> MVSGVGGSGGGRGGGRGGEEEPSSSHTPNNRRGGEQAQSSGTKSLRPRSNTESMSKAIQQYTVDARLHAVFEQSGESGKSFDYSQSLKTTTYGSSVPEQQITAYLSRIQRGGYIQPFGCMIAVDESSFRIIGYSENAREMLGIMPQSVPTLEKPEILAMGTDVRSLFTSSSSILLERAFVAREITLLNPVWIHSKNTGKPFYAILHRIDVGVVIDLEPARTEDPALSIAGAVQSQKLAVRAISQLQALPGGDIKLLCDTVVESVRDLTGYDRVMVHKFHEDEHGEVVAESKRDDLEPYIGLHYPATDIPQASRFLFKQNRVRMIVDCNATPVLVVQDDRLTQSMCLVGSTLRAPHGCHSQYMANMGSIASLAMAVIINGNEDDGSNVASGRSSMRLWGLVVCHHTSSRCIPFPLRYACEFLMQAFGLQLNMELQLALQMSEKRVLRTQTLLCDMLLRDSPAGIVTQSPSIMDLVKCDGAAFLYHGKYYPLGVAPSEVQIKDVVEWLLANHADSTGLSTDSLGDAGYPGA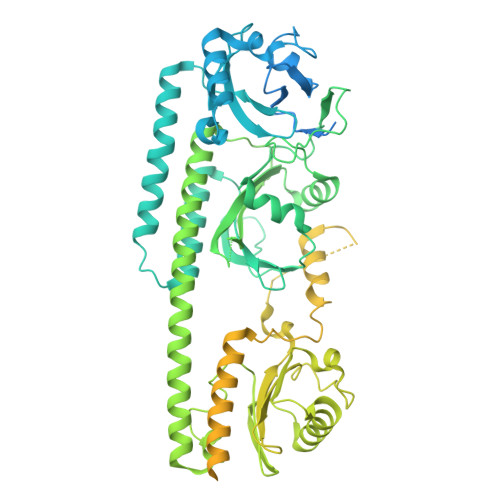AALGDAVCGMAVAYITKRDFLFWFRSHTAKEIKWGGAKHHPEDKDDGQRMHPRSSFQAFLEVVKSRSQPWETAEMDAIHSLQLILRDSFKESEAAMNSKVVDGVVQPCRDMAGEQGIDELGAVAREMVRLIETATVPIFAVDAGGCINGWNAKIAELTGLSVEEAMGKSLVSDLIYKENEATVNKLLSRALRGDEEKNVEVKLKTFSPELQGKAVFVVVNACSSKDYLNNIVGVCFVGQDVTSQKIVMDKFINIQGDYKAIVHSPNPLIPPIFAADENTCCLEWNMAMEKLTGWSRSEVIGKMIVGEVFGSCCMLKGPDALTKFMIVLHNAIGGQDTDKFPFPFFDRNGKFVQALLTANKRVSLEGKVIGAFCFLQIP2'-DEOXY-8-OXOGUANOSINE | 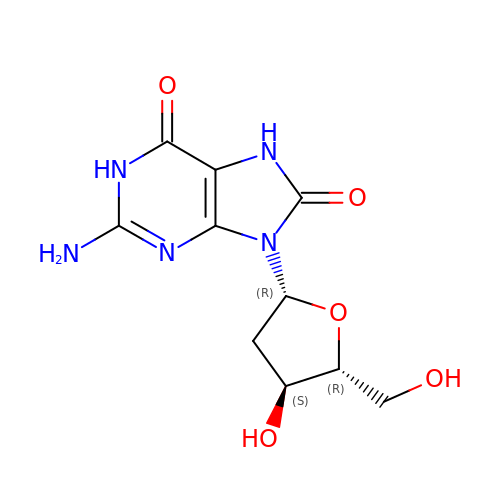C10 H13 N5 O5 | HCAJQHYUCKICQH-VPENINKCSA-N(2E,4R,5S)-2,3,4,5-TETRAHYDROXY-6-(PALMITOYLOXY)HEX-2-ENOIC 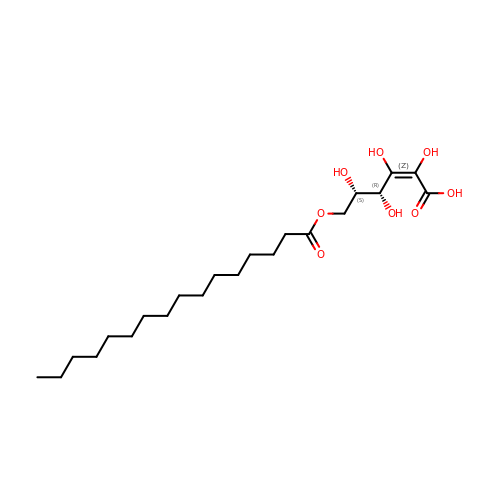ACID | C22 H40 O8 | XWTWKBKNEMLBKW-KCWNHAIFSA-N>[2x]MVISEKVRKALNDQLNREIYSSYLYLSMATYFDAEGFKGFAHWMKKQAQEELTHAMKFYEYIYERGGRVELEAIEKPPSNWNGIKDAFEAALKHEEFVTQSIYNILELAS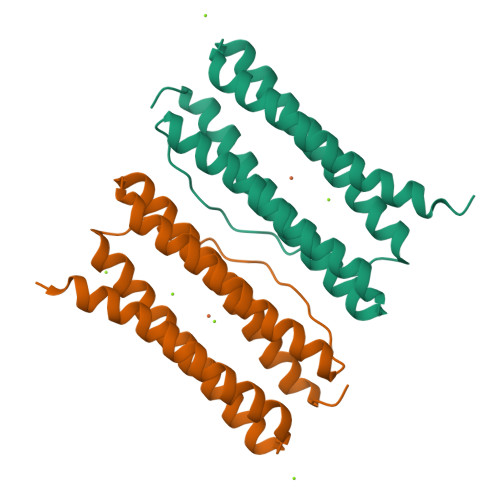EEKDHATVSFLKWFVDEQVEEEDQVREILDLLEKANG> SANNPWTGFQIFLSPYYANEVAAAAKQITDPTLSSKAASVANIPTFTWLDSVAKIPDLGTYLASASALGKSTGTKQLVQIVIYDLPDRDCAAKASNGEFSIANNGQANYENYIDQIVAQIQQFPDVRVVAVIEPDSLANLVTNLNVQKCANAKTTYLASVNYALTNLAKVGVYMYM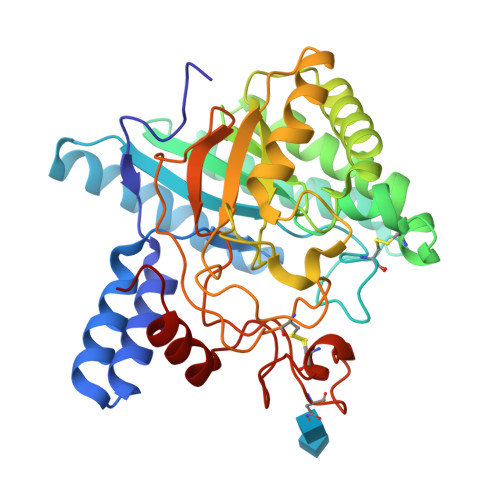DAGHAGWLGWPANLSPAAQLFTQVWQNAGKSPFIKGLATNVANYNALQAASPDPITQGNPNYDEIHYINALAPLLQQAGWDATFIVDQGRSGVQNIRQQWGDWCNIKGAGFGTRPTTNTGSQFIDSIVWVKPGGESNGTSNSSSPRYDSTCSLPDAAQPAPEAGTWFQAYFQTLVSAANPPL> EAAFWGASNELLHDPTMIKEGSSWYALGTGLTEERGLRVLKSSDAKNWTVQKSIFTTPLSWWSNYVPNYGQNQWAPDIQYYNGKYWLYYS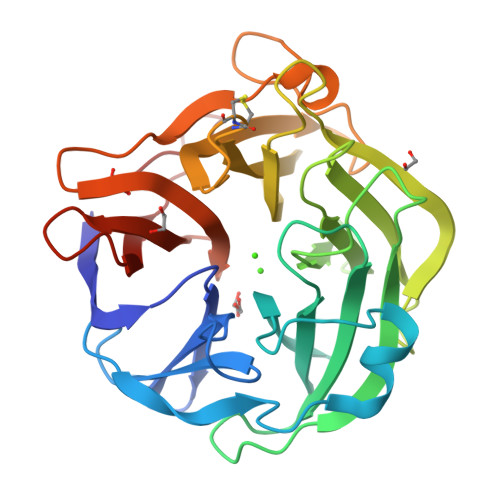VSSFGSNTSAIGLASSTSISSGGWKDEGLVIRSTSSNNYNAIDPELTFDKDGNPWLAFGSFWSGIKLTKLDKSTMKPTGSLYSIAARPNNGGALEAPTLTYQNGYYYLMVSFDKCCDGVNSTYKIAYGRSKSITGPYLDKSGKSMLEGGGTILDSGNDQWKGPGGQDIVNGNILVRHAYDANDNGIPKLLINDLNWSSGWPSY>[2x]MHGKLIGVGVGPGDSELLTLRAVNVLRSVPVIC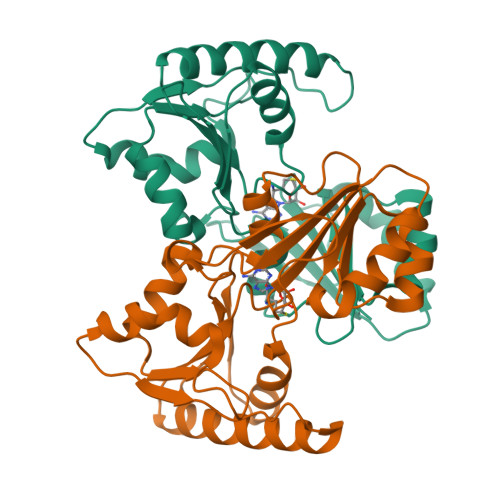APRSSSERESIALSIVEDILTERRDGCRILDPVFPMTDDRDELESHWDSAARMVAAELEDGRDVAFITLGDPSIYSTFSYLQQRIEDMGFKTEMVPGVTSFTACAATAGRTLVEGDEILLVVPRVDDRFERVLRDVDACVIMKTSRHGRRAMEVVESDPRGKDVVSVANCSMDDEVVERGFASGGGYLATTLVRFREQS>[4x]CG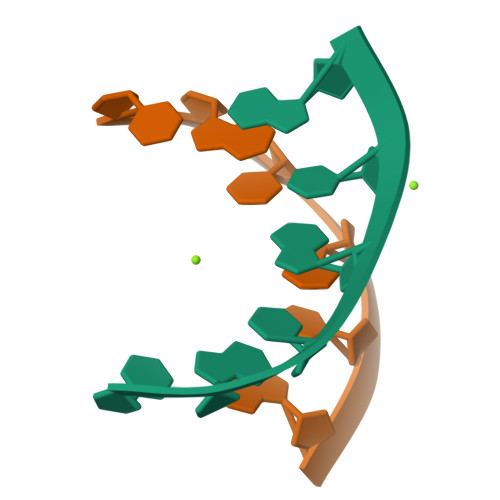CGXG> LALEADLRGAIGRGEITPYFQPIVRLSTGALSGFEALARWIHPRRGMLPPDEFLPLIEEMGLMSELGAHMMHA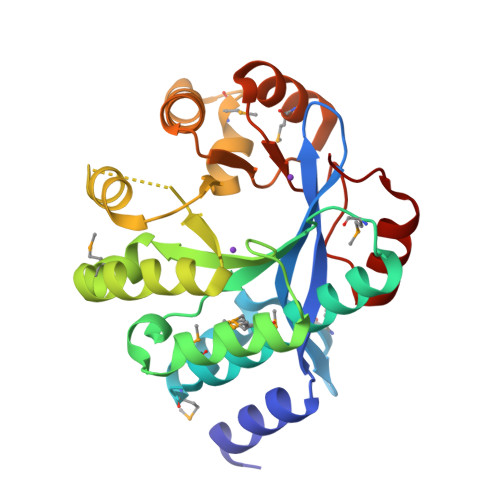AAQQLSTWRAAHPAMGNLTVSVNLSTGEIDRPGLVADVAETLRVNRLPRGALKLEVTESDIMRDPERAAVILKTLRDAGAGLALDDFGTGFSSLSYLTRLPFDTLKIDRYFVRTMGNNAGSAKIVRSVVKLGQDLDLEVVAEGVENAEMAHALQSLGCDYGQGFGYAPALSPQEAEVYLNEAYVDG[(1R)-1-{[6-(3-chloro-4-methylphenyl)thieno[2,3-d]pyrimidin-4-yl]amino}-2-(3-fluorophenyl)ethyl]phosphonic 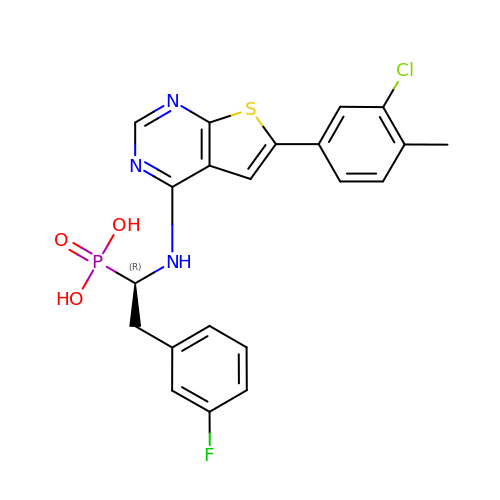acid | C21 H18 Cl F N3 O3 P S | ZSPBSSJYWQDARC-LJQANCHMSA-N>GDLADRFAELERRYDARLGVYVPATGTTAAIEYRADERFAFCSTFKAPLVAAVLHQNPLTHLDKLITYTSDDIRSYSPVAQQHVQTGMTIGQLCDAAIRYGDGTAANLLLADLGGPGGGTAAFTGYLRSLGDTVSRLDAEEPELNRDPPGDERDTTTPHAIALVLQQLVLGNALPPDKRALLTDWMARNTTGAKRIRAGFPADWKVIDKTGTGDYGRANDIAVVWSPTGVPYVVAVMSDRAGGGYDAEPREALLAEAATCVAGVLA[2x]

Here, we investigate how epistatic interactions influence the phenotypes of the two double mutant variants I105Y‐S130G and I105G‐G132N of Mycobacterium tuberculosis class A β‐lactamase, BlaC, which previously showed greatly improved fitness against the combination of carbenicillin and inhibitor, clavulanic acid, in a cellular assay (Radojković & Ubbink, 2024). The residue at position 105, known as “gatekeeper” (Feiler et al., 2013), is in most class A β‐lactamases an amino acid with an aromatic side chain, which yields high activity against penicillin‐like β‐lactams (Doucet et al., 2004; Judge et al., 2023; Papp‐Wallace et al., 2010). Ser130 is a conserved residue among class A β‐lactamases and plays an important role in substrate binding and proton transfer during β‐lactam ring opening (Atanasov et al., 2000; Helfand et al., 2003). The mutation S130G leads to the loss of activity for β‐lactam antibiotics and to slower inactivation of the enzyme by clavulanic acid (Egesborg et al., 2015).

The protein crystals of the I105Y‐S130G enzyme diffracted to 1.3‐Å resolution with R work/R free factor values of 14% and 17%. Two enzyme molecules were modeled in a unit cell with multiple residues adopting two conformations. The double conformation of the 127–130 backbone loop, harboring the mutation site, could be modeled in both chains, whereas loops containing the residues 213–216 and 86–91 could be modeled in two orientations only in one of the chains (respectively). The side chains of numerous other residues were also modeled in double conformations, including Ser70 and Tyr105. The comparison between the crystal structures of BlaC wild‐type and I105Y‐S130G revealed two differences in the active site. First, the substitution of Ile to Tyr at position 105 considerably widens access to the active site, due to the orientation of the Tyr side chain, which resembles the conformation found in the TEM‐1 enzyme (Strynadka et al., 1992). Second, in the place of the missing Ser130 side chain in BlaC I105Y‐S130G, an acetate ion is present, suggesting possible anion‐assisted substrate hydrolysis. The overall configuration looks similar to that of the wild‐type, with the acetate molecule occupying the position of the missing Ser130 side chain and engaging in H‐bonding with Ser70, Lys73, and Lys234. Our kinetic data indicate that acetate ions could potentially also take over this role, as the 4‐fold increase in acetate concentration augmented I105Y‐S130G activity by 64%. The enzyme either exhibits dynamic behavior on a faster timescale (ns−1) or the observed double conformations are present only in the crystals, for example, induced by the moderately low pH in the crystallization buffer (pH 4.5).>MSEELIKENMHMKLYMEGTVDNHHFKCTSEGEGKPYEGTQTMRIKVVEGGPLPFAFDILATSFLYGSKTFINHTQGIPDFFKQSFPEGFTWERVTTYEDGGVLTATQDTSLQDGCLIYNVKIRGVNFTSNGPVMQKKTLGWEAFTETLYPADGGLEGRNDMALKLVGGSHLIANIKTTYRSKKPAKNLKMPGVYYVDY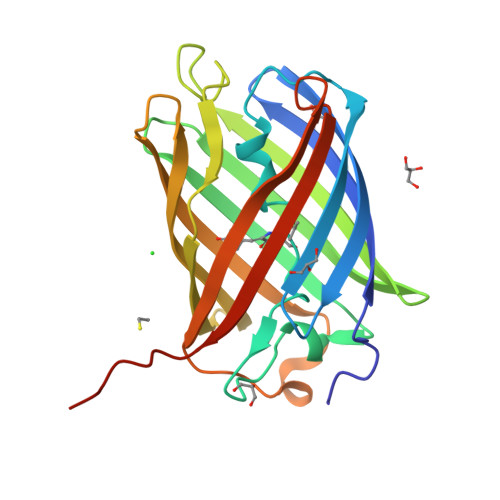RLERIKEANNETYVEQHEVAVARYCDLPSKLGHKLN[4x]> MSRRPTLRLGLDRDVYNIVLNLEQQGTDENGKRPRLTVDYVYDTIKRSNSSLARQKKRMLEDSIERVLAVRKEQAKAEEETDSDDLIEAQERERERQKAAQAQRDANLLNRQIAKSWGFASSPGAKAADGEKGTDTGSIATPAPATPAVAENMAADTPTTSTGPVLPASSTDRQPNGEPRPKKRKAAPKEIDRTPPTKVSILDIAGVDDTLQRLLKEVWFPLRGGEACEKMGYRYDNGVLLHGPSGCGKTTLAHAIAGSIGVAFIPVSAPSVIGGTSGESEKNIRDVFDEAIRLAPCLIFLDQIDAIAGRRESANKGMESRIVAEIMNGMDRIRQNTPLGKNVVVLAATNRPEFLDPAIRRRFSVEIDMGMPSERAREQILRSLTRDLSLADDINFKELAKMTPGYVGSDLQYVVKAAVSESFQANIDSLLAQARAKHPADHLANVSQPQRDWLLLEAHRDEEVSWPSTKITMEQFRKAVSLVQPASKREGFSTIPDTTWSHVGALEDVRKKLEMSIIGPIKNPELFTRVGIKPAAGILLWGPPGCGKTLVAKAVANESKANFISIKGPELLNKYVGESERAVRQLFSRAKSSAPCILFFDQMDALVPRRDDSLSDASARVVNTLLTELDGVGDRSGIYVIGATNRPDMIDEAIRRPGRLGTSIYVGLPSAEDRVKILKTLYRNTVKAP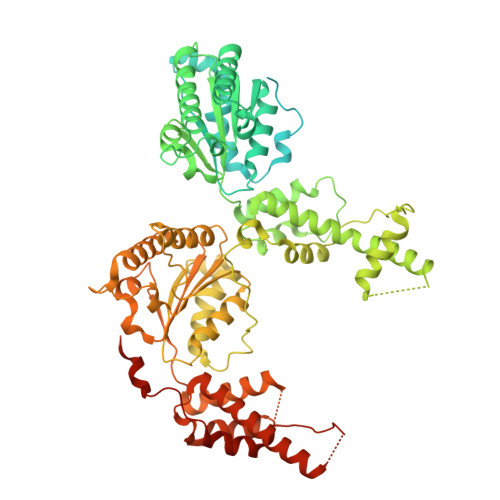KKREGTNGEDVDMTDAAAEQQHQGTTDADLEKVALDLRCTGFSGADLGNLMQAAAQACLERVYTQRQQKRKEGGSVAEEEEIEPVITMEDWEKALNEVKPSVKDPEKYMHSGFAAALEHHHHHH> MGCGGTADKNPAGNNGDSAKPAETKSGDSVSLTLRHINVRDTAKNTLALLEKVVKKTEAEVPGATFKLDGVEDTVNRDVKLKAEMAAGKPPQIFNLFGGADTQNYAKAGHLLPLNDILKELGLEDKFFELREFTVDGKIYGLPEAGFVEGFYYNTKLFADAGITSAPKTWDEFTKALEALKAKNITPIALGGGSGDGWAINMLANSLFVATAGPEAQEGFAKGTTKWTDPAVLDGFKRLKDLKDKGYIDPNVLGLKYSEGQAKFYTGQAAMLFDGSWATSAILDKDKSTVKDNVGYF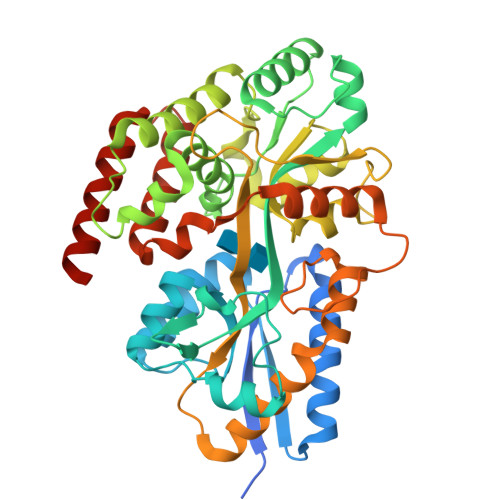RFPNIGGKGDNLINGGWSNGYGFSSHLNDAEKKAVKAFIKNFYTLEIQGEALGRDNRVPSMKGVPTPAEAAPLTKAIGEAQASAKAAFPAFDALVQPKVKVTLEQSVQELLGGQLTPEKLVEKMQKVQDEANAGKLEHHHHHH Within this class of proteins, the bromodomain and extraterminal domain (BET) family contains four members that are transcriptional coregulators and that recognize acetyllysines (AcKs) using a tandem pair of highly homologous bromodomains (BDs). Despite heavy academic and industry investment in this area, the generation of paralog-selective inhibitors has proved elusive because of the extremely high sequence similarity between the bromodomains of family members (90 to 95% within the acetyllysine-binding pocket residues). Using the highly conserved BET BDs as a model system, we conducted three mRNA display-based RaPID (random nonstandard peptides integrated discovery) screens using a single library (which contains >1012 unique members). Crystal structures of 13 distinct peptide–bromodomain complexes revealed highly diverse structures and binding modes among the cyclic peptide ligands.

Likewise, the most abundant family identified in the BRD3-BD2 selection (BRD3-BD2 family 3, accounting for 53% of total sequencing reads recovered for the top 500 peptides, including 3.2C) was not found in the BRD3-BD1 screen. On the other hand, the family to which 3.2B belongs was identified in the BRD3-BD1 screen with a relatively high abundance (BRD3-BD2 family 2, accounting for 8% of total sequencing reads recovered for the top 500 peptides from the BRD3-BD2 selection and 19% from the BRD3-BD1 selection; SI Appendix, Figs. S9B and S10). Cyclic peptide 3.2B showed strong binding but relatively little specificity, consistent with the abundance of related peptides found in the BRD3-BD1 selection; interactions with each of the six BDs had affinities in the range of ∼10 to 30 nM. Strikingly, 3.2B forms a single, well-defined α-helix in both structures; this helix contacts the AcK-binding surface of the two BDs with a very similar overall geometry and places its single AcK (AcK7) into the canonical binding pocket. It is notable that the AcK side chain enters the pocket at a similar diagonal angle to that observed for AcK5 in the peptide 3.1B binding to the “second” copy of BRD4-BD1. Because of this insertion angle, the hydrogen bond made by 3.2B with the pocket Asn is again mediated by a water molecule. Most of these hydrophobic contacts are conserved between the BRD2-BD1 and BRD4-BD2 structures, consistent with the similar affinities observed for the two interactions. Furthermore, peptides that belong to the same family but were derived from different selections (3.2B and 4.2A) adopted near-identical structures and binding modes.

> QGPLGSSKVSEQLKCCSGILKEMFAKKHAAYAWPFYKPVDVEALGLHDYCDIIKHPMDMSTIKSKLEAREYRDAQEFGADVRLMFSNCYKYNPPDHEVVAMARKLQDVFEMRFAKMPDEPEEP;> XWSWLCKKYNLIH Epoxide hydrolases (EHs, EC 3.3.2.9) are enzymes that catalyze the in vivo hydrolysis of an epoxide ring to the corresponding vicinal diols. Two novel EH enzymes of the α/β fold class have been identified from metagenomic samples from diverse locations in Russia and China. The nucleophile Asp102 in Sibe-EH (Asp101 in CH65-EH), is complemented by His277 and Asp249 (His270 and Asp241) to form a catalytic triad.

The ORF found in the Chinese metagenomic DNA sample (CH65-eh) consists of 879 nucleotides and encodes for a protein (CH65-EH) of 293 amino acids. The Sibe-EH showed the behavior of a moderately thermophilic enzyme with an apparent TM of 55°C, while CH65-EH showed higher thermal stability with an apparent TM of 85°C, which is, to our knowledge, the highest TM recorded for a wild-type EH to date. CH65-EH forms a dimer in solution according to its elution profile on the size exclusion chromatography column and in the crystal structure, as suggested by PISA. Within the formation of the dimer of CH65-EH 1,090 Å2 or 9% of the available surface area of the monomers is buried. The dimer interface is formed by the cap domains of the two monomers as shown in Figure 7. The interactions on the dimer interface are mainly hydrophobic although several H-bonds are also formed upon dimer formation. When analyzing the structures of the enzymes the higher thermostability of CH65-EH appears to result from a significant amount of hydrophobic interactions on the dimer interface and a higher proportion of secondary structure in this enzyme (56.8%) as calculated by PROMOTIF. In the case of CH65-EH and Sibe-EH the entrance to the active site cavity as seen in B. megaterium EH is totally obstructed by the adjacent monomer in the CH65-EH dimer and by a very different conformation in Sibe-EH in the region of residues 159–180. Instead, there is a separate small active site entrance funnel on the other side of protein monomer. The position of this funnel is approximately the same in CH65-EH and Sibe-EH, although it appears significantly more occluded in the CH65-EH enzyme.

>[2x]MNEMLKHEYVKVNGIKMHYVTQGKGKLLLLLHGFPDFWYVWRFQIPALAKHFRVVAPDLRGYNETDKPEGVENYRLDLLAKDILGLIKALGEEHAVVVGHDWGGIISWTLTAFNPQAVEKLVILNAPHPKAYMTRTKNSLRQLQKSWYVFFFQVANIPEKILSRNEFAFLKNMLIQSFVRRDLLTEEDLRIYVDAWSKSGALTSALNYYRANLNPDIIFSEKTVVFPKIKVPTLVIWGEKDVAISKDLIVNMEDFIEAPYSIKYFPECGHWVQLEEPELVRKHIEEFILKSDIHHHHHH> MGNLAGIMHRPDSEMAYVVNEQTVNIRLRTAKDDIVSVELLAGDPYSLRSLPTDEKFYQVPKQMTKIMSDGISDFWQVTVTEPKRRLAYAFLVTDMLGIQKIYSDKGFFKVADADLMDMNFYFRMPFFQTIDQYNAPEWVTDTVWYQIFPERFANGDVSNDPVGTKPWDSTDHPGREDFYGGDLQGILDHLDHLQELGISGIYLNPIFQAPSNHKYDTQDYMTVDPHFGDAKLFKQLVQAAHERGIRVMLDAVFNHIGDKSVQWQDVLKNEQASPYADWFHIHQFPATYTPTDNFEFAADATYDTFDYTPHMPKLNTSNPEVVDYLLNIATYWVKEFDIDAWRLDVANEIDHHFWRKFHDAMMALKPDFYILGQIWHTSQSWLVGDEFTAVMNYSYTGAILQYFLENESADALVQKMSHQLMLYRDATNRMMFNTVDS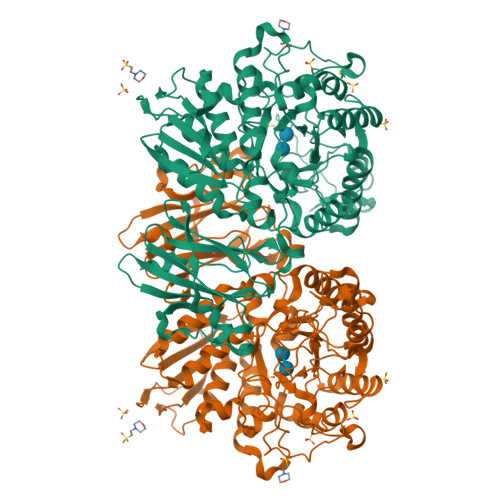HDTPRLMTLAHEDKQLAKSILTFTFMQPGVPSIYYGTEYGMTGENDPDDRKPMVWQPELQDHDLYDFMQKLVQVRRQVIAKLSDDKIIFDVIGERQIRLTREDNQTRIVGVFNNGTTDLTVAQPTSILLKTNQSETQLAPNDFMIWTEPVR Kinesins are a family of microtubule-based motors that play important roles in intracellular transport and cell division. Kinesin-1 transports cargo within cells, a process tightly coupled with ATP hydrolysis. Whereas kinesin-1 in solution is mostly loaded with ADP, ADP release is accelerated several thousand-fold upon microtubule binding. Here we characterized kinesin-1 P-loop mutations that interfere with ADP binding and determined the structure of the corresponding mutated nucleotide-free kinesins.

We also found that when T92 is mutated to a valine, the nucleotide content of this mutant was very low compared with that of wild-type kinesin. Together with the observation that the T92V fluorescence does not increase upon incubation with mant-ADP, these data indicate that T92V has lost most of the kinesin affinity for ADP. Using these T87A crystals as seeds, we were also able to crystallize wild-type apo-kinesin-1 and the T92V mutant and to determine their structures. Whereas most of the following analysis was performed taking the apo-T87A structure as a reference, identical conclusions could be reached from these wild-type apo-kinesin and T92V isomorphous structures. Taken together, these observations suggest that the P-loop destabilization in nucleotide-free T87A, as well as in the isomorphous structure of wild-type apo-kinesin and of T92V, is the combined result of ADP release and of the loss of the T87-E236 interactions.

>MADLAESNIKVMCRFRPLNESEVNRGDKYIAKFQGEDTVVIASKPYAFDRVFQSSTSQEQVYNDAAKKIVKDVLEGYNGTIFAYGQTSSGKVHTMEGKLHDPEGMGIIPRIVQDIFNYIYSMDENLEFHIKVSYFEIYLDKIRDLLDVSKTNLSVHEDKNRVPYVKGATERFVSSPDEVMDTIDEGKSNRHVAVTNMNEHSSRSHSIFLINVKQENTQTEQKLSGKLYLVDLAGSEKVSKTGAEGAVLDEAKNINKSLSALGNVISALAEGSTYVPYRDSKMTRILQDSLGGNARTTIVICCSPSSYNESETKSTLLFGQRAKTI[6x]> MATVTSVPGVYIEEDASPAMSVSASATAVPLFVARFTPLKPELAGVITRIGSWLDYTILFDSNVPSSARVTVSSTAVEPSPEFDALETASSKATTTYTYQIDDTEVVDPTASVALRLYFQNGGGPCYLYPLEKADDNGPLAALPDLIDEVGEITLLASPDPDETYRTAVYGALAASLDQHKGYFLLADSVN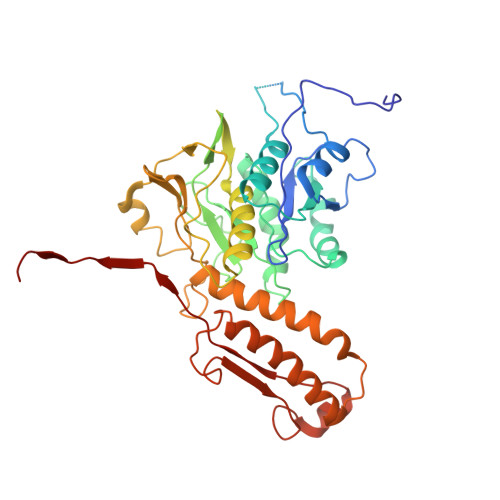GDAPSAVGGSAQVAVYYPNVEVPHTRKLDDAEVAIDGYLDDEGKAVTTLAALRVVNTEFAGEIAQSLSGDLSAPLSLPPSALIAGVYGKTDGERGVWKAPANVVLNGVSDVSVRVTNEQQAELNPKGINVIRHFSDRGLVVWGSRTQKDDDDWRYIPVRRLFDAAERDIKKALQPMVFEPNSQLTWKRVQTAIDNYLYRLWQQGALAGNKAEEAYFVRVGKGITMTQDEINQGKMIIQVGMAAVRPAEFIILKFTQDMSQ> MGESERSEAFGIPRDSPLSSGDAAELEQLRREAAVLREQLENAVGSHAPTRSARDIHQLEARIDSLAARNSKLMETLKEARQQLLALREEVDRLGQPPSGYGVLLATHDDDTVDVFTSGRKMRLTCSPNIDAASLKKGQTVRLNEALTVVEAGTFEAVGEISTLREILADGHRALVVGHADEERVVWLADPLIAEDLPDGLPEALNDDTRPRKLRPGDSLLVDTKAGYAFERIPKAEVEDLVLEEVPDVSYADIGGLSRQIEQIRDAVELPFLHKELYREYSLRPPKGVLLYGPPGCGKTLIAKAVANSLAKKMAEVRGDDAHEAKSYFLNIKGPELLNKFVGETERHIRLIFQRAREKASEGTPVIVFFDEMDSIFRTRGTGVSSDVETTVVPQLLSEIDGVEGLENVIVIGAS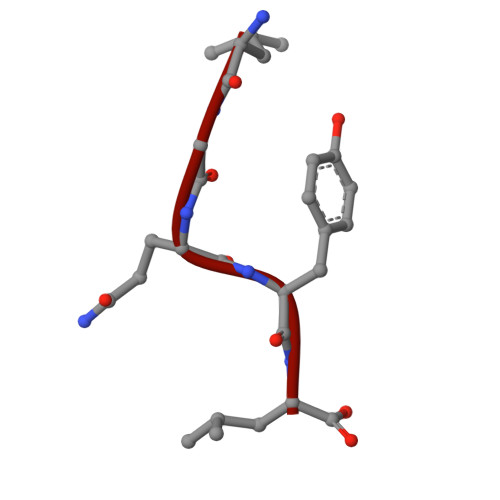NREDMIDPAILRPGRLDVKIKIERPDAEAAQDIYSKYLTEFLPVHADDLAEFDGDRSACIKAMIEKVVDRMYAEIDDNRFLEVTYANGDKEVMYFKDFNSGAMIQNVVDRAKKNAIKSVLETGQPGLRIQHLLDSIVDEFAENEDLPNTTNPDDWARISGKKGERIVYIRTLVTGKSSSASRAIDTESNLGQYL> 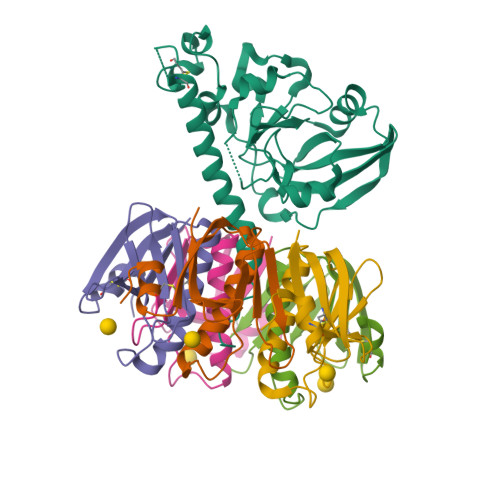NDDKLYRADSRPPDEIKQSGGLMPRGQSEYFDRGTQMNINLYDHARGTQTGFVRHDDGYVSTSISLRSAHLVGQTILSGHSTYYIYVIATAPNMFNVNDVLGAYSPHPDEQEVSALGGIPYSQIYGWYRVHFGVLDEQLHRNRGYRDRYYSNLDIAPAADGYGLAGFPPEHRAWREEPWIHHAPPGCGNAPRSSMSNTCDEKTQSLGVKFLDEYQSKVKRQIFSGYQSDIDTHNRIKDEL;>[5x]TPQNITDLCAEYHNTQIHTLNDKIFSYTESLAGKREMAIITFKNGATFQVEVPGSQHIDSQKKAIERMKDTLRIAYLTEAKVEKLCVWNNKTPHAIAAISMAN> SSQIRQNYSTEVEAAVNRLVNLYLRASYTYLSLGFYFDRDDVALEGVCHFFRELAEE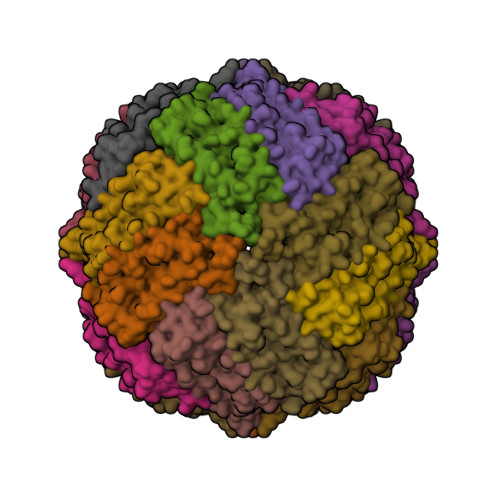KREGAERLLKMQNQRGGRALFQDLQKPSQDEWGTTLDAMKAAIVLEKSLNQALLDLHALGAAQADPHLCDFLESHFLDEEVKLIKKMGDHLTNIQRLVGSQAGLGEYLFERLTLKHD> GAMDADLAATTSREDFRLLAAEHRVVPVTRKVLADSETPLSAYRKLAANRPGTFLLESAENGRSWSRWSFIGAGAPTALTVREGQAVWLGAVPKDAPTGGDPLRALQVTLELLATADRQSEPGLPPLSGGMVGFFAYDMVRRLERLPERAVDDLCLPDMLLLLATDVAAVDHHEGTITLIANAVNWNGTDERVDWAYDDAVARLDVMTAALGQPLPSTVATFSRPEPRHRAQRTVEEYGAIVEYLVDQIAAGEAFQVVPSQRFEMDTDVDPIDVYRILRVTNPSPYMYLLQVPNSDGAVD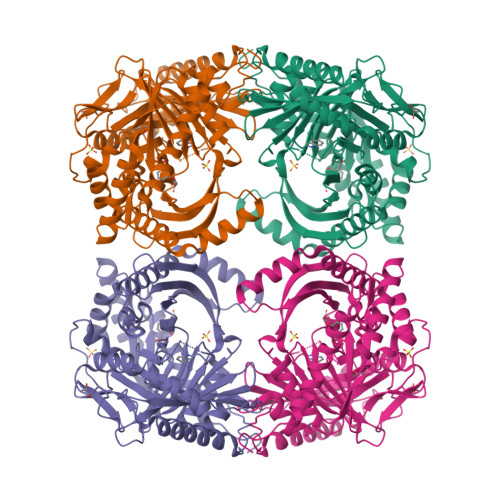FSIVGSSPEALVTVHEGWATTHPIAGTRWRGRTDDEDVLLEKELLADDKERAEHLMLVDLGRNDLGRVCTPGTVRVEDYSHIERYSHVMHLVSTVTGKLGEGRTALDAVTACFPAGTLSGAPKVRAMELIEEVEKTRRGLYGGVVGYLDFAGNADFAIAIRTALMRNGTAYVQAGGGVVADSNGSYEYNEARNKARAVLNAIAAAETLAAPGA> VIDRLVVQTSSGPVRGRSVTVQGREVHVYTGIPYAKPPVEDLRFRKPVPAEPWHGVLDATGLSATCVQERYEYFPGFSGEEIWNPNTNVSEDCLYINVWAPAKARLRHGRGANGGEHPNGKQADTDHLIHNGNPQNTTNGLPILIWIYGGGFMTGSATLDIYNADIMAAVGNVIVASFQYRVGAFGFLHLAPEMPSEFAEEAPGNVGLWDQALAIRWLKDNAHAFGGNPEWMTLFGESAGSSSVNAQLMSPVTRGLVKRGMMQSGTMNAPWSHMTSEKAVEIGKALINDCNCNASMLKTNPAHVMSCMRSVDAKTISVQQWNSYSGILSFPSAPTIDGAFLPADPMTLMKTADLKDYDILMGNVRDEGTYFLLYDFIDYFDKDDATALPRDKYLEIMNNIFGKATQAEREAIIFQYTSWEGNPGYQNQQQIGRAVGDHFFTCPTNEYAQALAERGASVHYYYFTHRTSTSLWGEWMGVLHGDEIEYFFGQPLNNSLQYRPVERELGKRMLSAVIEFAKTGNPAQDGEEWPNFSKEDPVYYIFSTDDKIEKLARGPLAARCSFWNDYLPKVRSWAGTCDGDS

Acetylcholinesterase (AChE) terminates synaptic transmissions at cholinergic synapses by rapid hydrolysis of the neurotransmitter, acetylcholine. The first X-ray structure of an insect AChE was published almost 20 years ago, and was that of the fruit fly Drosophila melanogaster. However, the active-site gorge is much smaller, with a volume ca. 50% of that of the vertebrate AChEs, due to the presence of additional aromatic residues. Thus, we here present optimized structures of DmAChE in its native form and in complexes with ZA and ZAI.

Two datasets collected from a single crystal of native DmAChE (100 images at high resolution and 100 images at low resolution) were processed and merged using XDS. The resolution of the data improved from 2.7 to 2.45 Å, and the number of unique reflections increased by 33% without dramatic loss of completeness (98.8% to 95.3%) or I/σ ratio (5.8 to 3.3) in the highest-resolution shell. Surprisingly, the R-free value of the native enzyme increased from 0.270 to 0.295. However, as calculated by Phenix, the R-free is slightly smaller than the R-work in the original structure of the native enzyme, which is abnormal and suggests a bias. It is noteworthy that the original statistics reported by Harel et al., R-work = 0.258 and R-free = 0.301, are in better agreement with the statistics of the updated native DmAChE structure. The resolution improved from 2.7 to 2.5 Å, the number of unique reflections increased by 25% without any loss of completeness (98.7% to 98.4%), and with an acceptable loss in I/σ ratio in the highest-resolution shell (5.8 to 3.3). These statistics indicate a clear improvement of the overall data quality for both crystals, with more information available for the refinement of the models.> GAEVGRLRYPPEMPGAEVKVYKKVDNVDLKLYIYKPADWKPADRRSAIVFFFGGGWQSGSPAQFRPQCEYFAGRGMVAMAADYRVGSRHNVKVADCVADAKSAIRWVRQHAAELGVDPQKIVASGGSAGGHLAACTVMVPDLEAPEEDHTISSQANAAILFNPVLILSREGLKDHVPRQDWEERLRERLGTEPKAVSPYHHIRAGLPPMIIFHGTADNTVPFETIRLFAEAMKKAGNRCELVPFEGAAHGFFNFGRGDNLAYQKTLELADEFLVEIGFLAPKGESQP

In order to facilitate the purification costs, we searched the ESTHER database for a thermophilic esterase, and identified the Esterase 2 from Thermogutta terrifontis (TtEst2) that has been previously structurally characterized, and presents an open active site that could ease protein engineering for further optimizations. The recombinant protein was purified, biochemically characterized, and its kinetic behavior towards different OPNA studied, before performing a structural analysis of its complexes formed when soaked in a racemic solution of the OPNA. Biophysical characterizations demonstrated that TtEst2 is a monomer in solution, with some polydispersity and good thermostability at physiological pH. We determined the bimolecular inhibition rate constants for five representative OPNA, namely tabun, sarin, cyclosarin, VX, and paraoxon, to estimate if this enzyme could scavenge them at a fast pace.

The orthorhombic crystals of TtEst2 of the uninhibited or apo state were obtained in conditions different that the ones previously reported by Sayer et al., where PEG 600 was used as a precipitating agent under microbatch conditions. A major difference can be observed compared to the model reported by Sayer et al. with the region comprising residues 172 to 181 that could not be modeled due to the absence of electron density. The region 165–190 is mostly disordered with high B-factors. Thus, these residues certainly explore a wider spatial range, and such dynamic disorder could explain the polydispersity of the solution measured by SEC-MALS, by mimicking multiple species. Tetrahedral-shaped electron density close to the active site was observed in a feature-enhanced map, and modeled as a sulfate molecule. However, in our apo structure, there was clearly no density allowing modeling of a whole HEPES molecule. The residues forming the catalytic triad are in an optimal configuration, with a 2.9 Å H-bond between Ser126 and His248, and a 2.9 Å H-bond between His248 and Asp216 (not shown). A water molecule sits at optimal H-bond distance between the catalytic serine, Ser126, and the main chain amide nitrogen atoms of residues Gly53 and Gly54 which form the oxyanion hole.> NYMGNPWTEYMAKYDIEEVHGSGIRVDLGEDAEVAGTQYRLPSGKCPVFGKGIIIENSNTTFLTPVATGNQYLKDGGFAFPPTEPLMSPMTLDEMRHFYKDNKYVKNLDELTLCSRHAGNMIPDNDKNSNYKYPAVYDDKDKKCHILYIAAQENNGPRYCNKDESKRNSMFCFRPAKDISFQNYTYLSKNVVDNWEKVCPRKNLQNAKFGLWVDGNCEDIPHVNEFPAIDLFECNKLVFE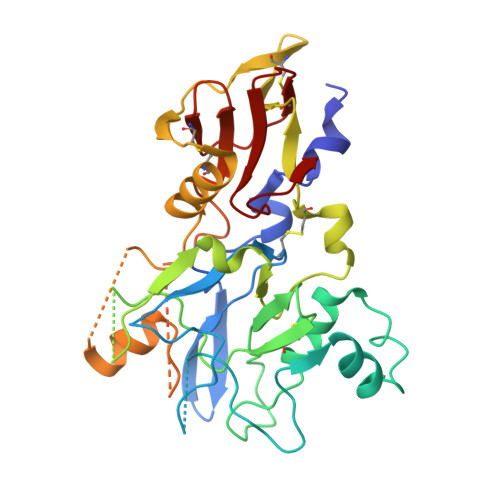LSASDQPKQYEQHLTDYEKIKEGFKNKNASMIKSAFLPTGAFKADRYKSHGKGYNWGNYNTETQKCEIFNVKPTCLINNSSYIATTALSHPIEVE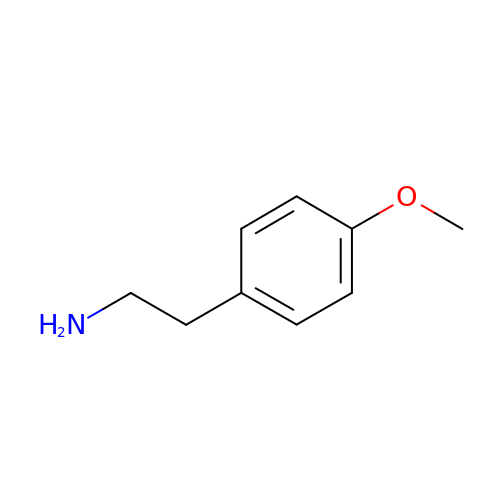2-(4-METHOXYPHENYL)ETHANAMINE | C9 H13 N O | LTPVSOCPYWDIFU-UHFFFAOYSA-N>MSVGIVYGDQYRQLCCSSPKFGDRYALVMDLINAYKLIPELSRVPPLQWDSPSRMYEAVTAFHSTEYVDALKKLQMLHCEEKELTADDELLMDSFSLNYDCPGFPSVFDYSLAAVQGSLAAASALICRHCEVVINWGGGWHHAKRSEASGFCYLNDIVLAIHRLVSSTPPETSPNRQTRVLYVDLDLHHGDGVEEAFWYSPRVVTFSVHHASPGFFPGTGTWNMVDNDKLPIFLNGAGRGRFSAFNLPL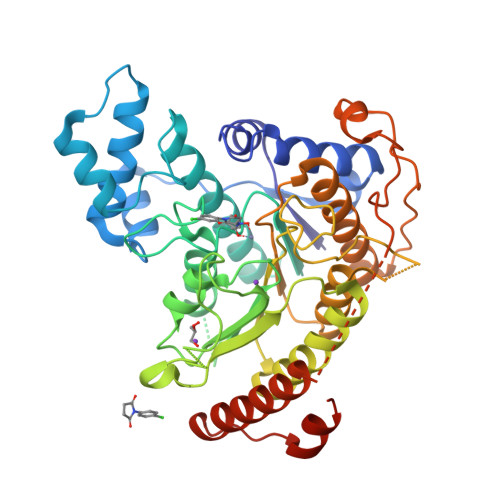EEGINDLDWSNAIGPILDSLNIVIQPSYVVVQCGADCLATDPHRIFRLTNFYPNLNLDSDCDSECSLSGYLYAIKKILSWKVPTLILGGGGYNFPDTARLWTRVTALTIEEVKGKKMTISPEIPEHSYFSRYGPDFELDIDYFPHESHNKTLDSIQKHHRRILEQLRNYADLNKLIYDYDQVYQLYNLTGMGSLVPR[4x]> MATLSLT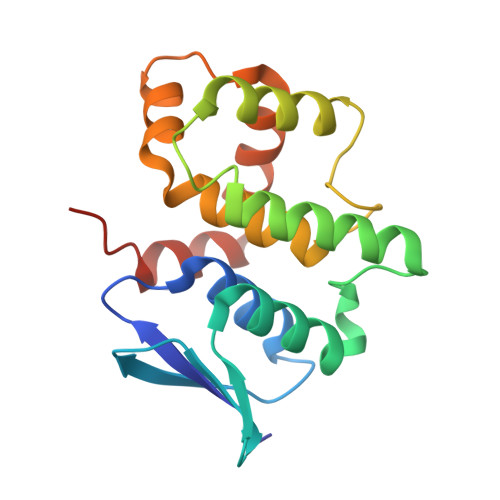VNSGDPPLGALLAVEHVKDDVSISVEEGKENILHVSENVIFTDVNSILRYLARVATTAGLYGSNLMEHTEIDHWLEFSATKLSSSDSFTSTINELNHSLSLRTYLVGNSLSLADLSVWATLKGNAAWQEQLKQKKAPVHVKRWFGFLEAQQAFQSVGTKWDVSTTKAR3-bromo-5-[(4-pyrrolidin-1-ylpiperidin-1-yl)carbonyl]pyridine | C15 H20 Br N3 O | 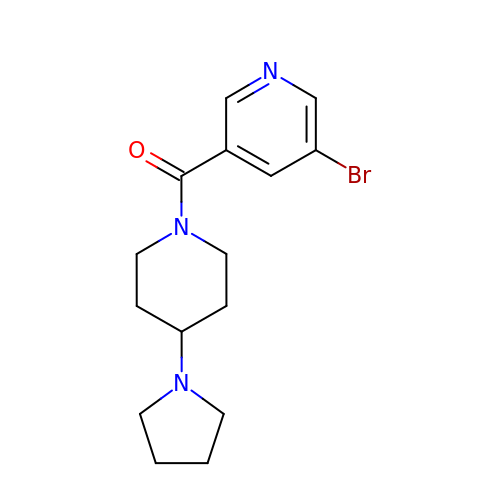CQERVFFAOOUFEQ-UHFFFAOYSA-N>[2x]MPATHHSSATSAERPTVVGRIPVLDVRPVVQRGRRPAKAVTGESFEVSATVFREGHDAVGANVVLRDPRGRPGPWTPMRELAPGTDRWGATVTAGETGTWSYTVEAWGDPVTTWRHHARIKIPAGLDTDLVLEEGARLYERAAADVPGREDRRELLAAVDALRDESRPAASRLAAALTPQVDAVLARHPLRDLVTSSDPLPLLVERERALYG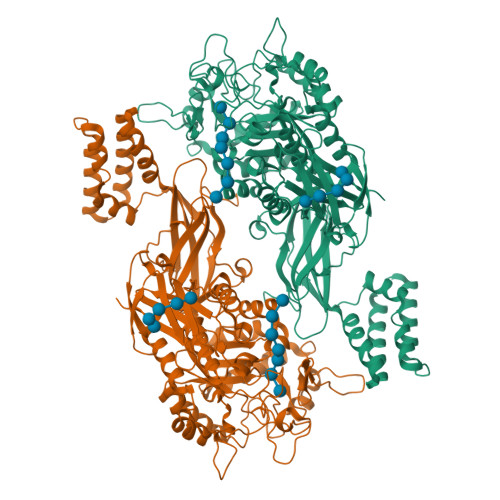AWYEFFPRSEGTPHTPHGTFRTAARRLPAIAAMGFDVVYLPPIHPIGTTHRKGRNNTLSATGDDVGVPWAIGSPEGGHDSIHPALGTLDDFDHFVTEAGKLGLEIALDFALQCSPDHPWVHKHPEWFHHRPDGTIAHAENPPKKYQDIYPIAFDADPDGLATETVRILRHWMDHGVRIFRVDNPHTKPVAFWERVIADINGTDPDVIFLAAAFTRPAMMATLAQIGFQQSYTYFTWRNTKQELTEYLTELSGEAASYMRPNFFANTPDILHAYLQHGGRPAFEVRAVLAATLSPTWGIYSGYELCENTPLREGSEEYLDSEKYQLKPRDWTRAAREGTTIAPLVTRLNTIRRENPALRQLRDLHFHPTDKEEVIAYSKRQGSNTVLVVVNLDPRHTQEATVSLDMPQLGLDWHESVPVRDELTGETYHWGRANYVRLEPGRTPAHVCTVLRPSHPQIGGSHTT>MN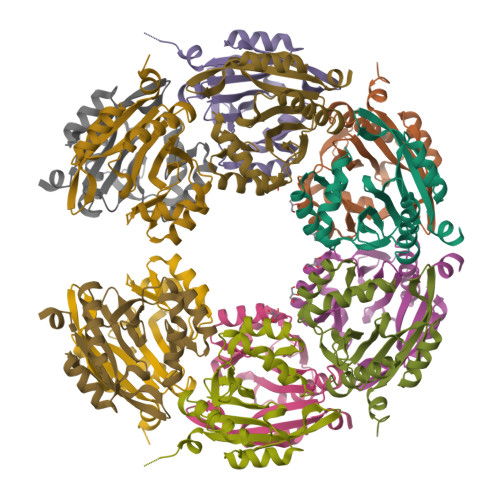SQLTLRALERGDLRFIHNLNNNRNIMSYWFQEPYESFDQLEELYNKHIHDNAERRFVVEDAQKNLIGLVELIEINYIHRSAEFQIIIAPEHQGKGFARTLINRALDYSFTILNLHKIYLHVAVENPKAVHLYEECGFVEEGHLVEEFFINGRYQDVKRMYILQSKYLNRSE[6x]> MVIPYVIEQTARGERVYDIYSRLLKDRIIFLGTPIDAQVANVVVAQLLFLDAQNPNQEIKLYINSPGGEVDAGLAIYDTMQFVRAPVSTIVIGMAASMAAVILAAGEKGRRYALPHAKVMIHQPWGGVRGTASDIAIQAQEILKAKKLLNEILAKHTGQPLEK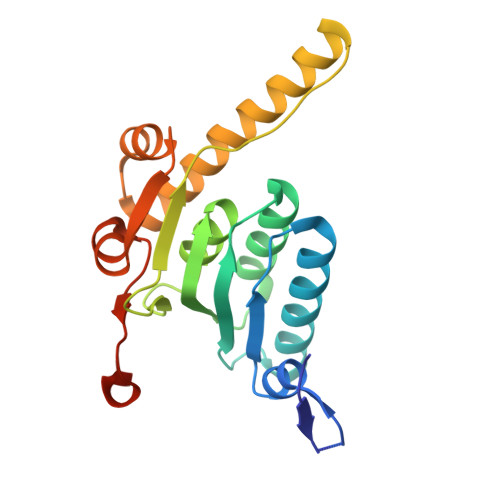VEKDTDRDYYLSAQEALEYGLIDQVVTREEALEHHHHHHHH> MGKKSPDSSQGASGPA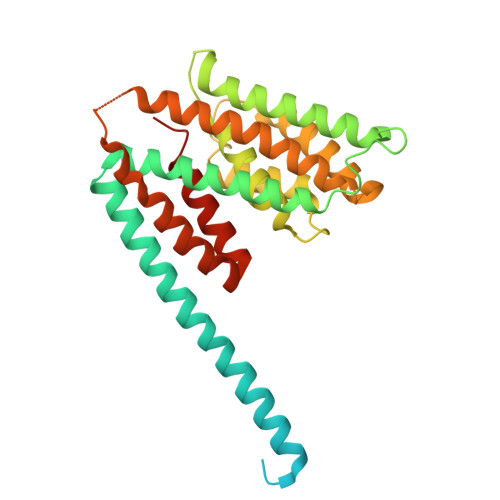MQSPSGPTIRPTRPAPPPPTTGGANAKRPATHGKGRAPQPPTAGSSSGSEQPTAMSSEVAKLVSELKDAVHSHAESQKVLKKVSQELQTKWTDWENNRGPDYLLHGYRVIARALQQTYTEQSMLIEGTSSTGPVPQAVTVAKDAVTQTVRGAIKNLENPKPGNDPDGVLMQVVISLGIEGPTLDPGESIQNFLETRVSDFGGDDSDIDYTSDIARLGSALDRVRENHPNEMPRIWIALARELGAAVHSHATSVRIANAGKNHTRDVVRMANESSRLLQGMKVLSVGAWANTMTVLIGDLFEHHHHHHHHH3-[(2S,4aR,6R,7R,7aS)-2,7-dihydroxy-2-oxotetrahydro-2H,4H-2lambda~5~-furo[3,2-d][1,3,2]dioxaphosphinin-6-yl]-6-phenyl-3,4-dihydro-9H-imidazo[1,2-a]purin-9-one | C18 H16 N5 O7 P | 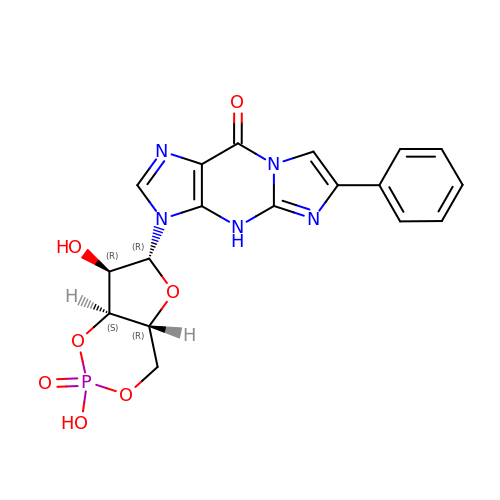TVSIKYJKUPRIDV-LSCFUAHRSA-N>GSHMGEGEGVQLTAAQELMIQQLVAAQLQCNKRSFSDQPKVTPWPLGADPQSRDARQQRFAHFTELAIISVQEIVDFAKQVPGFLQLGREDQIALLKASTIEIMLLETARRYNHETECITFLKDFTYSKDDFHRAGLQVEFINPIFEFSRAMRRLGLDDAEYALLIAINIFSADRPNVQEPGRVEA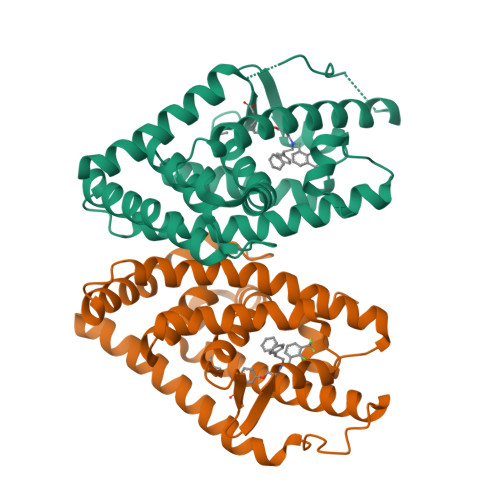LQQPYVEALLSYTRIKRPQDQLRFPRMLMKLVSLRTLSSVHSEQVFALRLQDKKLPPLLSEIWDVHE[4x]>APADNAADARPVDVSVSIFINKIYGVNTLEQTYKVDGYIVAQWTGKPRKTPGDKPLIVENTQIERWINNGLWVPALEFINVVGSPDTGNKRLMLFPDGRVIYNARFLGSFSNDMDFRLFPFDRQQFVLELEPFSYNNQQLRFSDIQVYTENIDNEEIDEWWIRGKASTHISDIRYDHLSSVQPNQNEFSRITVRIDAVRKIGYFVIQTYLPCIMTVILSQVSFWLNRESVPARTVFGVTTVLTMTTLSISARNSLPKVAYATAMDWFIAVCYAFVFSALIEFATVNY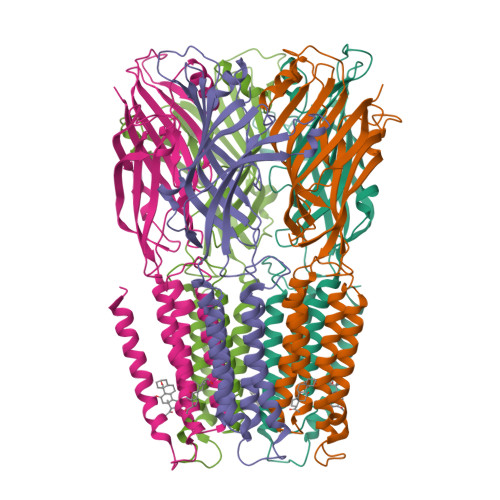FTKRGVESVSKIDRLSRIAFPLLFGIFNLVYWATYLN[10x]>[4x]MGKKNSKLKQDTIDRLTTDTYFTEKEIRQWHKGFLKDCPNGLLTEQGF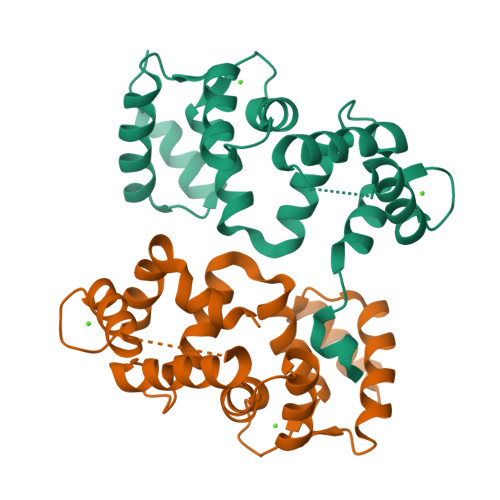IKIYKQFFPDGDPSKFASLVFRVFDENNDGAIEFEEFIRALSITSRGNLDEKLHWAFRLYDVDNDGYITREEMYNIVDAIYQMVGQQPQTEDENTPQKRVDKIFDQMDKNHDDRLTLEEFREGSKADPRMVQALSLGGD>MFGRKKGDVIDAGAELERAEQERIEGEYGASELASERRPHTPGARTLLMVLLCVIAVVLVTLSYKAYKVRGVVEDDDAQPQQVVRQVIPGYTPRPIRPEPENVPEPPQPTTSVPAIQPAPVTQPVRPQPTGPREKTPYELARERMLRSGLTAGSGGGEDLPRPQGGDVPAGGLMGGGGGGGELAEKLQPMRLSGSSAGRLGNRDMLITQGTQLDCVLETRLVTTQPGMTTCHLTRDVYSTSGRVVLLDRGSKVVGFYQGGLRQGQARIFVQWSRIETPSGVVINLDSPGTGPLGEAGLGGWIDRHFWERFGGAIMISLIGDLGDWASRQGSRQGDNSIQFSNTANGVESAAAEALRNSINIPPTLYKNQGERVNILVARDLDFSDVYSLESIPTK[16x];>MKKLAIVALLASLHAVPALALDVPSSSRYDHRIRYVTYNPADVVQVDTVLGVATHIMLEEGEQYLTHAFGDSEAYAFARKGRHIFIKPQAELANTNLIVVTDRRSYKFRL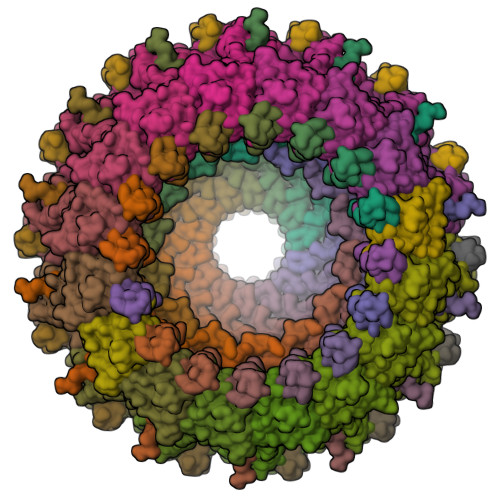QMRNDRNGAMYELAFRYPDTQARQTREANARAAVEAAFEQRVGAYYNLKYMMSGDKDIAPVNAWDDGRFTYFKFSANADLPSIYFVDAEGNESLVPRTTVGSSNNIIAVHKVNPKWMIRLGNRALAIFNEAYDPNGVPNDTGTASPAVRRVNKGGN[16x];>[14x]MKTIIFAILMTGLLSACASAPKPKQPSDFNREPVNKTVPVEIQRGAL>[2x]GSCNVEPVGRLHIFSGAHGPEKDFPLHLGKNVVGRMPDCSVALPFPSISKQHA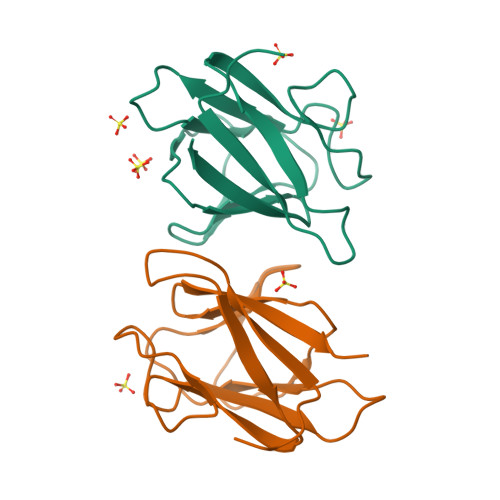EIEILAWDKAPILRDCGSLNGTQILRPPKVLSPGVSHRLRDQELILFADLLCQYHRLDVSLP>SELDPKGQHVCVASSPSAELQCCAGWRQKDQECTIPICEGPDACQKDEVCVKPGLCRCKPGFFGAHCSSRCPGQYWGPDCRESCPCHPHGQCEPATGACQCQADRWGARCEFPSRHHHH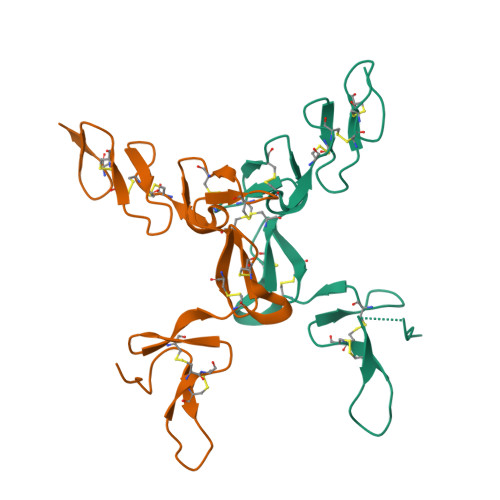HH[2x]>[2x]SHMDPVSVWGNTPLATVDPEIHDLIEKEKRRQCRGIELIASENFTSFAVIEA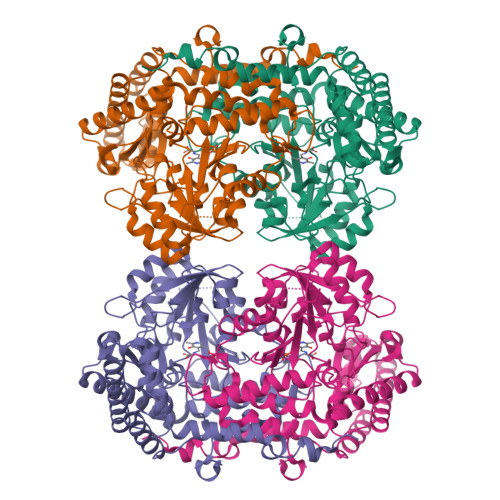LGSALTNKYSEGMPGNRYYGGNEYIDQIENLCRSRALQAFHLDAQSWGVNVQPYSGSPANFAAYTAVLNPHDRIMGLDLRSGGHLTHGYYTSGGKKISATSIYFESLPYKVNSTTGYIDYDRLEEKALDFRPKLIICGGSAYPRDWDYKRFREVADKCGALLLCDMAHTSGLVAAQEVNSPFEYCDIVTTTTHKSLRGPRAGMIFYRKGPKPPKKGQPENAVYDFEDKINFAVFPSLQGGPHNHQIGALAVALKQAASPGFKAYAKQVKANAVALGKYLMGKGYSLVTGGTENHLVLWDLRPLGLTGYKVEKLCDLCNITVNKNAVFGDSSALAPGGVRIGAPAMTSRGLVEKDFEQIGEFLHRAVTLTLEIQKEHGKLLKDFNKGLVNNKAIEDLKADVEKFSALFDMPGFLVSEMKYKD The protein studied in this work is pre-mRNA-splicing factor 16 (Prp16) and is required for the transition of the spliceosome from the C to the C* state. Therefore, Prp16 binds the 3′-end sequence of the intron RNA and translocates towards the spliceosome, leading to dissociation of the branching factors Yju2 and Cwc25 and thereby enabling exon ligation. Prp16 belongs to the DEAH-box proteins, which share a highly conserved helicase core formed by two RecA-like domains. All DEAH-box helicases have a common C-terminal domain architecture comprising winged-helix (WH), helix-bundle (HB) and oligosaccharide-binding fold (OB-fold) domains.

The spliceosomal DEAH-box helicase Prp16 from the thermo­philic ascomycete C. thermophilum (ctPrp16) was crystallized in complex with ADP to mimic a post-catalytic state. An N- and C-terminally truncated construct ctPrp16 (302–920) was used for crystallization, as the removed parts are expected to be mainly disordered according to the PredictProtein server. The reported structure of ctPrp16 in complex with ADP was determined at a resolution of 1.9 Å and was refined to an R work of 19.3% and an R free of 23.8%. The atomic model comprises ctPrp16 (302–920), one ADP molecule, one magnesium ion, one polyethylene glycol (PEG) molecule and 423 water molecules. The overall assembly of ctPrp16 can be divided into six different entities: the N-terminal extension (302–311), two RecA-like domains [referred to as RecA1 (312–468) and RecA2 (467–661)], the WH domain (662–728), the HB domain (729–842) and the OB-fold domain (843–920). In the structure reported here, an ADP molecule as well as the catalytically required magnesium ion are present at the interface between the RecA1 and RecA2 domains, corresponding to ctPrp16 in the post-catalytic state. The magnesium ion is hexavalently coordinated by four water molecules, Thr342 located within motif I and the β-phosphate of the ADP molecule. While Arg635 (motif VI) belongs to this conserved region of DEAH-box helicases, Thr593 and Asp595 do not. The adenine moiety does not form any polar contacts with ctPrp16 residues, but the adenine interacts with Phe567 via π–π stacking. While all other X-ray structures harbor the β-hairpin between the WH and OB-fold domains, independent of the nucleotide- or substrate-loading state, in ctPrp16 the upper part of the β-hairpin with its loop region is pushed out of the cleft and interacts exclusively with the OB-fold domain. However, this conformation appears to be an artifact caused by interaction with a symmetry mate within the crystal lattice. Superposition of the ctPrp16 structure with the structure of the ctPrp22–RNA complex shows that the conserved Lys is located virtually in the same position in both structures, meaning that RNA binding seems to be unaffected by the unique conformation of the β-hairpin in ctPrp16.

> GPLGSPNTLKEQREFLPAFAVREDLLRVIRDNQVVIVIGETGSGKTTQLTQFLYEDGYGKTGMIGCTQPRRVAAMSVAKRVAEEMEVKLGTLVGYAIRFEDCTSKETVIKYMTDGVLLRESLNEPDLDRYSCIIMDEAHERALNTDVLMGLFKKILQRRRDLKLIITSATMNSKRFSDFFGGAPEFTIPGRTFPVDILFHRSPVEDYVDQAVQQVLAIHVSKPAGDILVFMTGQEDIEVTCELIQERLAALNDPPKLSVLPIYSQMPADLQAKIFDRAPPGVRKCIVATNIAETSLTVDGIMYVVDCGYSKLKVYNPRMGMDTLQITPISQANAAQRAGRAGRTGPGQAYRLYTEKQFRDEMYMQTIPEIQRTNLSNTVLLLKSLGVKDLLDFDFMDPPPQDTITTSLYDLWALGALDNLGELTELGRKMNAFPMDPPLAKLLIMSEEYGCSEEMVTIVSMLSVPNVFYRPKERQEESDAAREKFFVPESDHLTYLHVYTQWKANGYSDAWCARHFLHSKSLRRAREVRDQLLDIMKMQHMRMVSCGTDWDIIRKCICSGYYHQAAKVKGIGEYINLRTSVTVQLHPTSALYGLGFLPDYVVYHELILTSKEYMSTVTAVDPHWLAELEPSAV> GSPRTVEEIFKDYSARRAALLRALTKDVDDFYSQCDPEKENLCLYGHPNESWEVNLPAEEVPPELPEPALGINFARDGMQRKDWLSLVAVHSDCWLLSVSFYFGARLNRNERKRLFSLINDLPTLFDV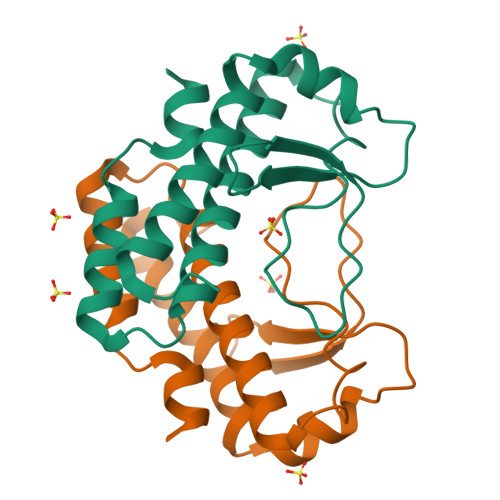VTGRKAM>[2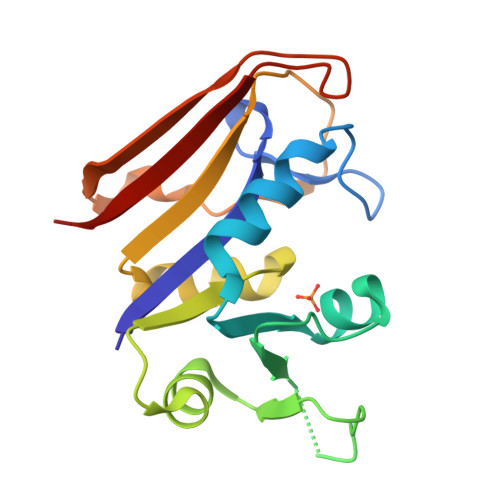x]MIVSMIAALANNRVIGLDNKMPWHLPAELQLFKRATLGKPIVMGRNTFESIGRPLPGRLNIVLSRQTDYQPEGVTVVATLEDAVVAAGDVEELMIIGGATIYNQCLAAADRLYLTHIELTTEGDTWFPDYEQYNWQEIEHESYAADDKNPHNYRFSLLERVK>[2x]SAQEPARKKQDPPVTHDLRVSLEEIYSGCTKKMKISHKRLNPDGKSIRNEDKILTIEVKKGWKEGTKITFPKEGDQTSNNIPADIVFVLKDKPHNIFKRDGSDVIY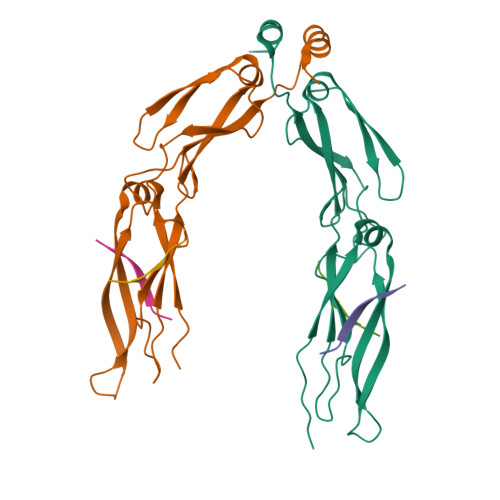PARISLREALCGCTVNVPTLDGRTIPVVFKDVIRPGMRRKVPGEGLPLPKTPEKRGDLIIEFEVIFPERIPQTSRTVLEQVLPI;>[4x]GPTIEEVD>[2x]MLHLLALFLHCLPLASGDYDICKSWVTTDEGPTWEFYACQPKVMRLKDYVKVKVEPSGITCGDPPERFCSHENPYLCSNECDASNPDLAHPPRLMFDKEEEGLATYWQSITWSRYPSP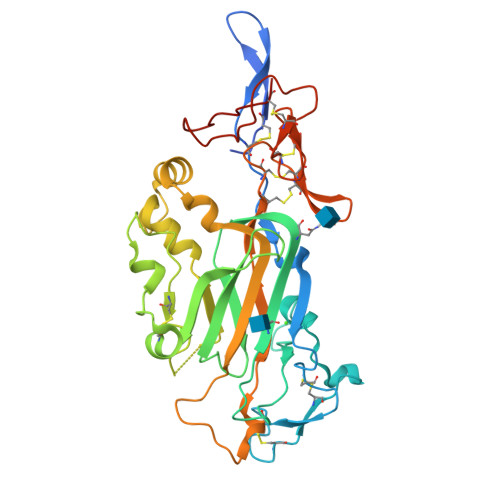LEANITLSWNKTVELTDDVVMTFEYGRPTVMVLEKSLDNGRTWQPYQFYAEDCMEAFGMSARRARDMSSSSAHRVLCTEEYSRWAGSKKEKHVRFEVRDRFAIFAGPDLRNMDNLYTRLESAKGLKEFFTLTDLRMRLLRPALGGTYVQRENLYKYFYAISNIEVIGRCKCNLHANLCSMREGSLQCECEHNTTGPDCGKCKKNFRTRSWRAGSYLPLPHGSPNACAGTHHHHHH>MSKTQEFRPLTLPPKLSLSDFNEFIQDIIRIVGSENVEVISSKDQIVDGSYMKPTHTHDPHHVMDQDYFLASAIVAPRNVADVQSIVGLANKFSFPLWPISIGRNSGYGGAAPRVSGSVVLDMGKNMNRVLEVNVEGAYCVVEPGVTYHDLHNYLEANNLRDKLWLDVPDLGGGSVLGNAVERGVGYTPYGDHWMMHSGMEVVLANGELLRTGMGALPDPKRPETMGLKPEDQPWSK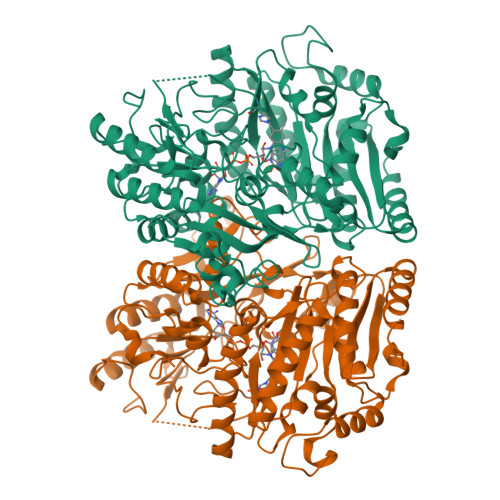IAHLFPYGFGPYIDGLFSQSNMGIVTKIGIWLMPNPRGYQSYLITLPKDGDLKQAVDIIRPLRLGMALQNVPTIRHILLDAAVLGDKRSYSSRTEPLSDEELDKIAKQLNLGRWNFYGALYGPEPIRRVLWETIKDAFSAIPGVKFYFPEDTPENSVLRVRDKTMQGIPTYDELKWIDWLPNGAHLFFSPIAKVSGEDAMMQYAVTKKRCQEAGLDFIGTFTVGMREMHHIVCIVFNKKDLIQKRKVQWLMRTLIDDCAANGWGEYRSHLAFMDQIMETYNWNNSSFLRFNEVLKNAVDPNGIIAPGKSGVWPSQYSHVTWKL[2x]>[2x]MQTQKPVFSEVTVHDPSIIKANGTYYVFGSHLASAKSTDLMNWTQISSSVHDGNPLIPNVYEELKETFEWAESDTLWAPDVTQLEDGKFYMYYNACRGDSPRSALGLAVADDIEGPYKNKGIFLKSGMDGISNDGTPYDATKHPNVVDPHTFFDQNGKLWMVYGSYSGGIFILEMDKKTGFPLPGQGYGKKLIGGNHSRIEGAYILYHPETQYYYLYMSFGGLAADGGYNIRVARSKNPDGPYY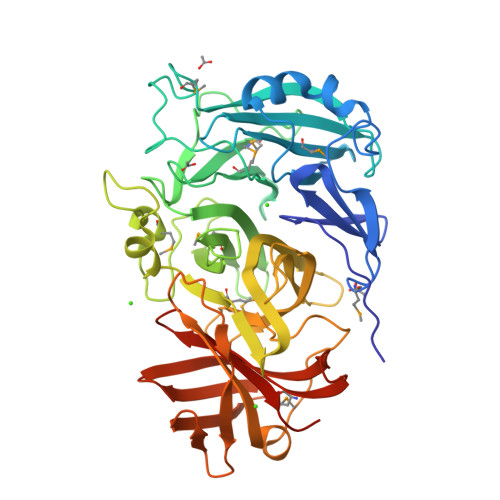DAEGHAMIDVRGKEGTLFDDRSIEPYGVKLMGNFSFNNKNGYVSPGHNSAFYDEKSGKSYLIFHTRFPGRGEEHEVRVHQLLMNKQGWPVVAPHRYAGEKLEKVKKSDVIGDYELVRHGKDISADIKESKEIRLNQNGKITGAVAGTWKNTGHNKIELKIDGKTYDGVFLRQWDAASERKVMTFSALSREGDAVWGSSLKRAEFLEHHHHHH> YGPKGPKGPKGKPGPDGDPG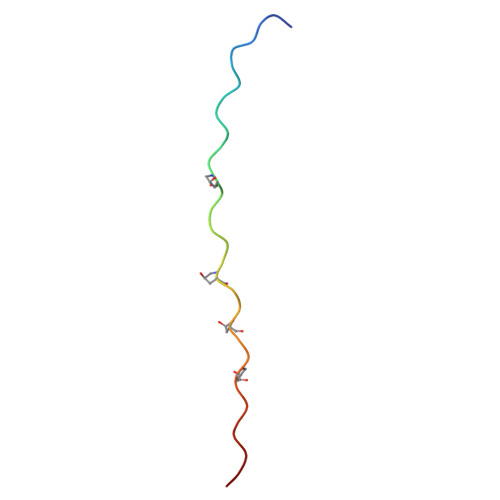DPGDPGPKGPKG In humans, the CALHM family encompasses six paralogs, some of which function as non-selective channels that are permeable to large substances such as ATP. We identified the three paralogs, CALHM2, 4 and 6, to be highly expressed in this organ. The CALHM subunits thus constitute unique modular building blocks that assemble with different stoichiometries into large membrane channels. In contrast to previously described CALHM structures, where the oligomeric state of individual channels was described as uniform, our data show heterogeneous populations with CALHM4 and CALHM6 assembling as decameric and undecameric channels with similar abundance and CALHM2 as predominantly undecameric proteins with a smaller population of dodecamers (Figure 3—figure supplements 2–4 and 6). Despite the unknown activating stimuli, our study has provided insight into gating transitions of CALHM channels by showing two conformations with either a cylindrical pore of uniform large dimeter within the membrane that is constricted at the intracellular side as in case of CALHM4 and a conical pore that continuously narrows from its extracellular entry towards the cytoplasm as in case of CALHM6.

As in case of CALHM4, data of CALHM6 shows a heterogeneous distribution of decameric and undecameric channels, but in this case with a prevalence of the former amounting to 60% of the classified particles. Both assemblies of CALHM6 contain subunits with equivalent conformations, which are better defined in the smaller oligomers. Unlike CALHM4, there is no dimerization of CALHM6 channels and the C-terminal region following the cytoplasmic helix CTH instead appears to engage in intramolecular interactions with the outside of the cytoplasmic rim for most of its length. Although the general organization of the CALHM6 channel closely resembles CALHM4, it shows a distinctly different state of the pore. Whereas in the cylindrical pore conformation of CALHM4, TM1 tightly interacts with TM3, which is a part of a densely packed outer rim of the pore consisting of TM2-4, the helix has dissociated from its interaction site and instead moved towards the symmetry axis to alter the pore geometry in the conical conformation of CALHM6. In a superposition of the subunits, similar conformations are observed for α-helices TM2 and 4 and the C-terminal helix CTH and larger differences in the interacting helices TM1 and 3. These differences are most pronounced for TM1, which in CALHM6 has detached from TM3 and moved by 60° towards the pore axis around a hinge located upstream of a conserved phenylalanine at the end of TM1. As a consequence of the disruption of its interaction with TM1, the intracellular halve of TM3 tilts away from the pore axis by 30° around a pivot located close to a conserved proline residue (P115 in CALHM4), which probably destabilizes the helix.

>[11x]MEKFRAVLDLHVKHHSALGYGLVTLLTAGGERIFSAVAFQCPCSAAWNLPYGLVFLLVPALALFLLGYVLSARTWRLLTGCCSSARASCGSALRGSLVCTQISAAAALAPLTWVAVALLGGAFYECAATGSAAFAQRLCLGRNRSCAAELPLVPCNQAKASDVQDLLKDLKAQSQVLGWILIAVVIIILLIFTSVTRCLSPVSFLQLKFWKIYLEQEQQILKSKATEHATELAKENIKCFFEGSHPKEYNTPSMKEWQQISSLYTFNPKGQYYSMLHKYVNRKEKTHSIRSTEGDTVIPVLGFVDSSGINSTPEL> VQAVAVLKGDAGVSGVVKFEQASESEPTTVSYEIAGNSPNAERGFHIFEFGDATNGCVSAGPHFNPFKKTHGAPTDEVRHVGDMGNVKTDENGVAKGS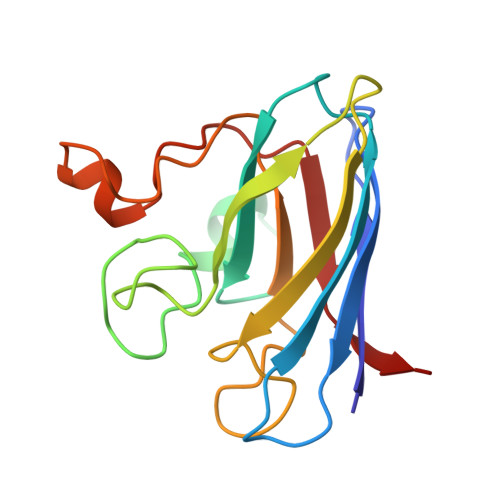FKDSLIKLIGPTSVVGRSVVIHAGQDDLGKGDTEESLKTGNAGPRPACGVIGLTN PYK (EC 2.7.1.40) forms a tetramer that catalyzes transfer of phosphate from phosphoenolpyruvate (PEP) to ADP to form pyruvate and ATP. MtbPYK adopts a tetrameric architecture formed by identical subunits with three domains (A, B and C domains), similar to typical PYK structures. The catalytic site is located in the cleft between the A and B domains (lid domain), while the C domain harbours a canonical AMP allosteric site. The allosteric site binding for G6P (sugar monophosphate site) is adjacent to the AMP site and lies between the A and C domains.

Unlike trypanosomatid PYKs that use additional salt bridges across the C–C interface to stabilise the R-state tetramer structure, the motions of the AC-cores in MtbPYK require the disruption of C–C interface interactions between the AMP loop and the C-terminal tail loop (Thr455…Asp470), as well as the hydrogen bonds (H-bonds) formed between the two adjacent Cα4 structures (Thr422…Asp423). To study this type of structural plasticity and to probe the mobile secondary structural elements (α helix, β strand, loops), we superposed monomers (instead of tetramers) of all available R-state MtbPYK structures onto the T-state monomer structure. We then further analysed the movements of superposed structures and found that Cα1 and Cα4 both rotated and shifted by ~6° from the T-state (yellow) to the fully ligated R-state (cyan). We propose a three-step ‘rock-shape-lock’ model to describe the synergistic allostery of MtbPYK: (1) Subunits of the MtbPYK tetramer rock 9° simultaneously from the T-state to the R-state in response to substrate binding, movements that are coupled with interface-loop interplay and catalytic-site formation via the movement of helices Aα6′ and Aα6.

>[4x]GGHMTRRGKIVCTLGPATQRDDLVRALVEAGMDVARMNFSHGDYDDHKVAYERVRVASDATGRAVGVLADLQGPKIRLGRFASGATHWAEGETVRITVGACEGSHDRVSTTYKRLAQDAVAGDRVLVDDGKVALVVDAVEGDDVVCTVVEGGPVSDNKGISLPGMNVTAPALSEKDIEDLTFALNLGVDMVALSFVRSPADVELVHEVMDRIGRRVPVIAKLEKPEAIDNLEAIVLAFDAVMVARGDLGVELPLEEVPLVQKRAIQMARENAKPVIVATQMLDSMIENSRPTRAEASDVANAVLDGADALMLSGETSVGKYPLAAVRTMSRIICAVEENSTAAPPLTHIPRTKRGVISYAARDIGERLDAKALVAFTQSGDTVRRLARLHTPLPLLAFTAWPEVRSQLAMTWGTETFIVPKMQSTDGMIRQVDKSLLELARYKRGDLVVIVAGAPPGTVGSTNLIHVHRIGEDDV> SNAMTDTYNSISNFIENELTALLSSDDYLMDDLAGELPNEVCRLLKAQVIEKRKDAMSRGKQDLLSKEIYDNESELRASQSQQIMELVGDIPKYSLGSELRNRVEGEPQSTSIERLIEDVLKLPQMEVADEEEVEVENDLKVLSEYSNLRKDLILKCQALQIGESKLSDILSQT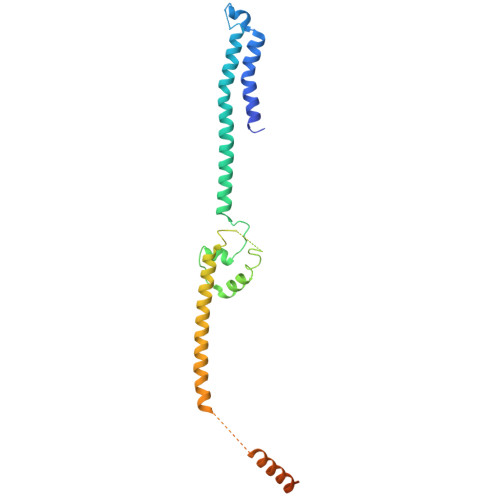NSINSLTTSIKEASEDDDISEYFATYNGKLVVALEEMKLLLEEAVKTFGNSPEKREKIKKILSELKK>GSAMGSSDEPRDDFKEAVNAFNPNPIEKWTGRFNTENASVRRRTLNVPGFKSIPTVYTEATLPLNKDVTDGRLTVVVNINTVQPFTRRTPLRVKREKWYTCSSSQCSGSSSKCDCHRKHDEFRNKCISEGGRYTTESSKCRLGEKCGYCKQNVYLATLYLVAGSVGGGMYRESDKYQSALYPFYDISQGYEPRQPSSVNVRLYSEGDPFIAFQQLTEGREEFGI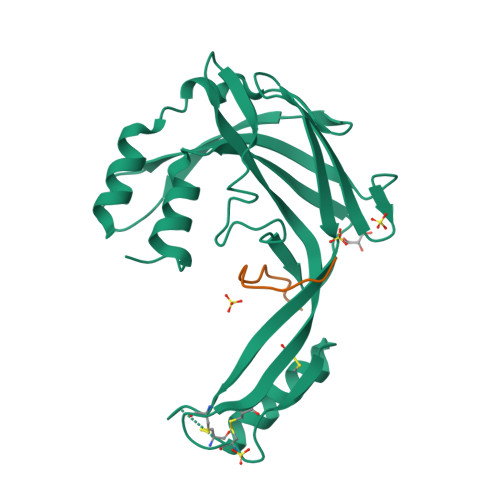PNRTVGAAA[4x]> MADTRIGVTIYKYDDCFMSVVRKAIEQDAKAAPDVQLLMNDSQNDQSKQNDQIDVLLAKGVKALAINLVDPAAAGTVIEKARGQNVPVVFFNKEPSRKALDSYDKAYYVGTDSKESGIIQGDLIAKHWAANQGWDLNKDGQIQFVLLKGEPGHPDAEART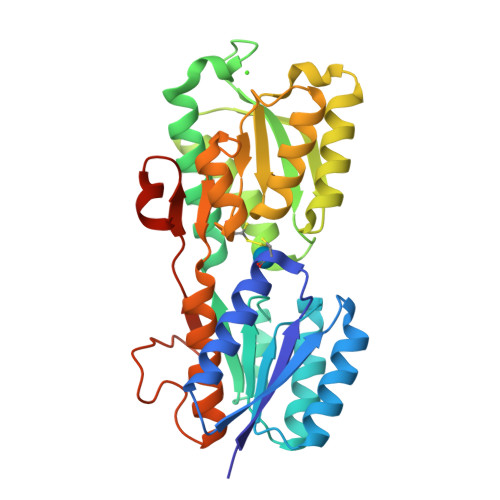TYVIKELNDKGIKTEQLQLDTAMWDTAQAKDKMDAWLSGPNANKIEVVIANNDAMAMGAVEALKAHNKSSIPVFGVDACPEALALVKSGALAGTVLNDANNQAKATFDLAKNLADGKGAADGTNWKIDNKVVRVPYVGVDKDNLAEFSKKGSHHHHHH> GSDPFSFLLNYSHCGTLVESSLNKGGMWCVPVSPVNLAAYTLQGEALVFNDAFVSKTHNWLHFMASTTAYWRGTLHYQMRVTYKDRNAACRNLVAFYTTNNESLFGFNNKPVGDTGISSVMGDSFSVDITVPFLIPTCYLQTIRGKFDYLNSCNGC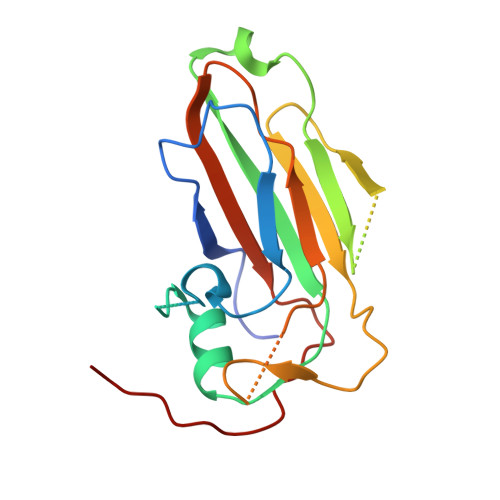IYFHLPTKSATSVQLWVRPGQDFDFARFRLLKAGYT>SQPVAITDGIYWVGAVDWNIRYFHGPAFSTHRGTTYNAYLIVDDKTALVDTVYEPFKEELIAKLKQIKDPVKLDYLVVNHTESDHAGAFPAIMELCPDAHVLCTQRAFDSLKAHYSHIDFNYTIVKTGTSVSLGKRSLTFIEAPMLHWPDSMFTYVPEEALLLPNDAFGQHIATSVRFDDQVDAGLIMDEAAKYYANILMPFSNLITKKLDEIQKINLAIKTIAPSHGIIWRKDPGRIIEAYARWAEGQGKAKAVIAYDTMWLSTEKMAHALMDGLVAGGCEVKLFKLSVSDRNDVIKEILDARAVLVGSPTINNDILPVVSPLLDDLVGLRPKNKVGLAFGAY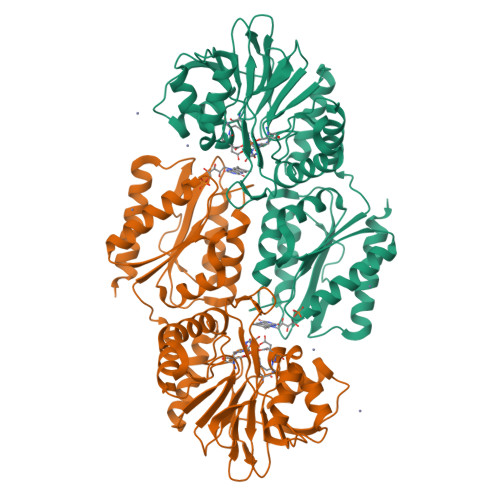GWGGGAQKILEERLKAAKIELIAEPGPTVQWVPRGEDLQRCYELGRKIAARIAD[4x]> DNINTLWTGVNPTEANCQIMNSSESNDCKL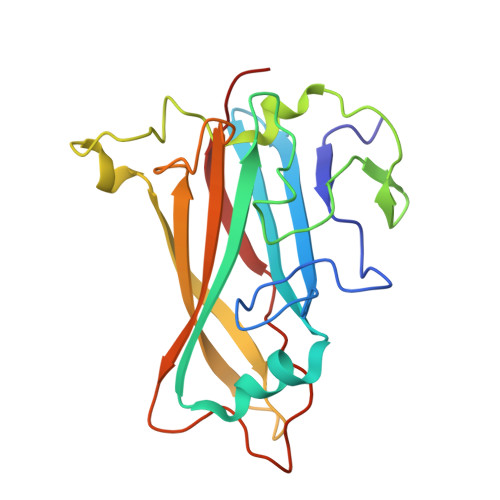ILTLVKTGALVTAFVYVIGVSNNFNMLTTHRNINFTAELFFDSTGNLLTRLSSLKTPLNHKSGQNMATGAITNAKGFMPSTTAYPFNDNSREKENYIYGTCYYTASDRTAFPIDISVMLNRRAINDETSYCIRITWSWNTGDAPEVQTSATTLVTSPFTFYYIREDD The Hermes DNA transposon is a member of the eukaryotic hAT superfamily, and its transposase forms a ring-shaped tetramer of dimers. The Hermes transposase is composed of 612 amino acids and is organized in four domains. Architecturally, the Hermes transposase is unusual as it spontaneously forms a ring-shaped tetramer of dimers. All hAT transposases are predicted to contain an N-terminal BED zinc-finger domain organized around a conserved CCHH or CCHC motif that coordinates Zn2+13, but no structural information is available for Hermes as the constructs used in previous structural work lacked the first 78 amino acids.

As we were unable to generate interpretable cryo-EM data for a single Hermes assembly that bound one LE and RE transposon end at the same time, we determined the structure of the transpososome bound to two REs. Using a similar approach as described for the LE-LE version based on partial signal subtraction to focus the reconstruction on the DNAs and the Hermes dimers A and C, a reconstruction at 5.1 Å resolution was obtained and a model could be generated. The 3D class that refined best clearly showed 5’-flanks synapsed in the top A1/A2 dimer revealing two parallel DNAs. In marked contrast to the LE-LE transpososome, none of the refined 3D classes showed density corresponding to either free or bound BED domains. The 3’-ends of 8 + RE-TIR + 30 DNAs were both inserted in the C1/C2 dimer in a TIR-like fashion, suggesting that this interaction was not a function of STR/BED interactions, but a possible consequence of the particular length of the DNA used. The cryo-EM structure of the core of the RE-RE transpososome showed that the RE does not interact with any BED domain, suggesting that RE binding relies on the interaction of its TIR with one dimer in the octamer, perhaps aided by nonspecific contributions from dimer C across the octamer. By contrast, the right-end is bound to no BED domains at all.

>[4x]MEKMDNLEVKAKINQGLYKITPRHKGTSFIWNVLADIQKEDDTLVEGWVFCRKCEKVLKYTTRQTSNLCRHKCCASLKQSRELKTVSADCKKEAIEKCAQWVVRDCRPFSAVSGSGFIDMIKFFIKVGAEYGEHVNVEELLPSPITLSRKVTSDAKEKKALISREIKSAVEKDGASATIDLWTDNYIKRNFLGVTLHYHENNELRDLILGLKSLDFERSTAENIYKKLKAIFSQFNVEDLSSIKFVTDRGANVVKSLANNIRINCSSHLLSNVLENSFEETPELNMPILACKNIVKYFKKANLQHRLRSSLKSECPTRWNSTYTMLRSILDNWESVIQILSEAGETQRIVHINKSIIQTMVNILDGFERIFKELQTCSSPSLCFVVPSILKVKEICSPDVGDVADIAKLKVNIIKNVRIIWEENLSIWHYTAFFFYPPALHMQQEKVAQIKEFCLSKMEDLELINRMSSFNELSATQLNQSDSNSHNSIDLTSHSKDISTTSFFFPQLTQNNSREPPVCPSDEFEFYRKEIVILSEDFKVMEWWNLNSKKYPKLSKLALSLLSIPASSAASERTFSLAGNIITEKRNRIGQQTVDSLLFLNSFYKNFCKLDI> MSEEFGGQ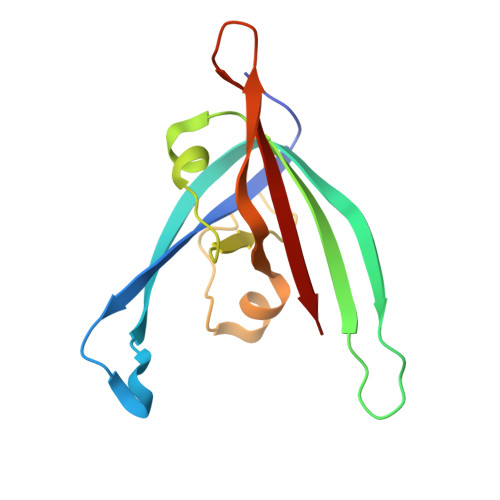VVALVSVAETGVPGWGGLKAKARTTTRQPGVHFRPASSTETPDGQTNVATEVWKLTAPPTAAVLAAKPGGELVYDGTEHPESLDLDSAAGRAATFRVDGPIMPKYDLAGQVHHVTIMCKRQAG>MGSSHHHHHHSQDPNSMPDNTIQWDKDADGIVTLTMDDPSGSTNVMNEAYIESMGKAVDRLVAEKDSITGVVVASAKKTFFAGGDVKTMIQARPEDAGDVFNTVETIKRQLRTLETLGKPVVAAINGAALGGGLEIALACHHRIAADVKGSQLGLPEVTLGLLPGGGGVTRTVRMFGIQNAFVSVLAQGTRFKPAKAKEIGLVDELVATVEELVPAAKAWIKEELKANPDGAGVQPWDKKGYKMPGGTPSSPGLAAILPSFPSNLRKQLKGAPMPAPRAILAAAVEGAQVDFDTASRIESRYFASLVTGQVAKNMMQAFFFDLQAINAGGSRPEGIGKTPIKRIGVLGAGMMGAGIAYVSAKAGYEVVLKDVSLEAAAKGKGYSEKLEAKALERGRTTQERSDALLARITPTADAADFKGVDFVIEAVFENQELKHKVFGEIEDIVEPNAILGSNTSTLPITGLATGVKRQEDFIGIHFFSPVDKMPLVEIIKGEKTSDEALARVFDYTLAIGKTPIVVNDSRGFFTSRVIGTFVNEALAMLGEGVEPASIEQAGSQAGYPAPPLQLSDELNLELMHKIAVATRKGVEDAGGTYQPHPAEAVVEKMIELGRSGRLKGAGFYEYADGKRSGLWPGLRETFKSGSSQPPLQDMIDRMLFAEALETQKCLDEGVLTSTADANIGSIMGIGFPPWTGGSAQFIVGYSGPAGTGKAAFVARARELAAAYGDRFLPPESLLS[2x];>MSEEAFIYEAIRTPRGKQKNGSLHEVKPLSLVVGLIDELRKRHPDLDENLISDVILGCVSPVGDQGGDIARAAVLASGMPVTSGGVQLNRFCASGLEAVNTAAQKVRSGWDDLVLAGGVESMSRVPMGSDGGAMGLDPATNYDVMFVPQSIGADLIATIEGFSREDVDAYALRSQQKAAEAWSGGYFAKSVVPVRDQNGLLILDHDEHMRPDTTKEGLAKLKPAFEGLAALGGFDDVALQKYHWVEKINHVHTGGNSSGIVDGAALVMIGSAAAGKLQGLTPRARIVATATSGADPVIMLTGPTPATRKVLDRAGLTVDDIDLFELNEAFASVVLKFQKDLNIPDEKLNVNGGAIAMGHPLGATGAMILGTMVDELERRNARRALITLCIGGGMGVATIIERV[2x]

The Mycobacterium tuberculosis trifunctional enzyme (MtTFE) is an α2β2 tetrameric enzyme in which the α-chain harbors the 2E-enoyl-CoA hydratase (ECH) and 3S-hydroxyacyl-CoA dehydrogenase (HAD) active sites, and the β-chain provides the 3-ketoacyl-CoA thiolase (KAT) active site. Linear, medium-chain and long-chain 2E-enoyl-CoA molecules are the preferred substrates of MtTFE. Mtb is capable of switching its metabolic preference during the latent stage of infection in order to utilize host-derived fatty acids as a source of carbon rather than glucose or glycerol. The Mtb genome encodes an unusually large set of enzymes of the β-oxidation cycle; however, only a single trifunctional enzyme (MtTFE) that catalyzes three of the last four reactions in the β-oxidation cycle is present in Mtb, in contrast to other bacteria such as Escherichia coli, which has two TFEs. Here, 226 fragments were screened in a crystallographic fragment-binding study of MtTFE crystals, resulting in the structures of 16 MtTFE–fragment complexes.

14 (out of 16) of the characterized MtTFE–fragment complexes involve compounds with aromatic rings [the only exceptions are fragment M-1 (the anion) and fragment B-B3 (trehalose)].> MSLIFLDYDGTLVPIIMNPEESYADAGLLSLISDLKERFDTYIVTGRSPEEISRFLPLDINMICYHGACSKINGQIVYNNGSDRFLGVFDRIYEDTRSWVSDFPGLRIYRKNLAVLYHLGLMGADMKPKLRSRIEEIARIFGVETYYGKMIIELRVPGVNKGSAIRSVRGERPAIIAGDDATDEAAFEANDDALTIKVGEGETHAKFHVADYIEMRKILKFIEMLGVQ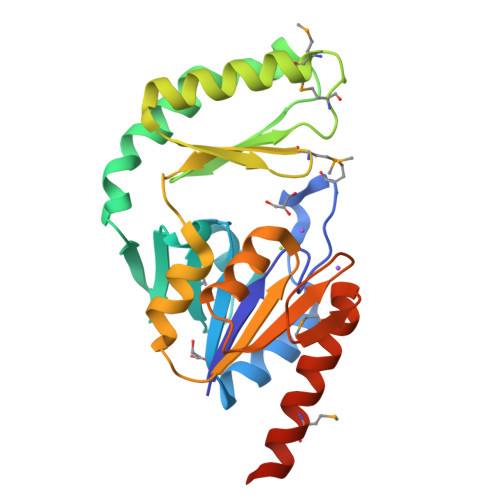KKQEGHHHHHH N-[1-(2,6-dimethoxybenzyl)piperidin-4-yl]-4-sulfanylbutanamide | C18 H28 N2 O3 S | 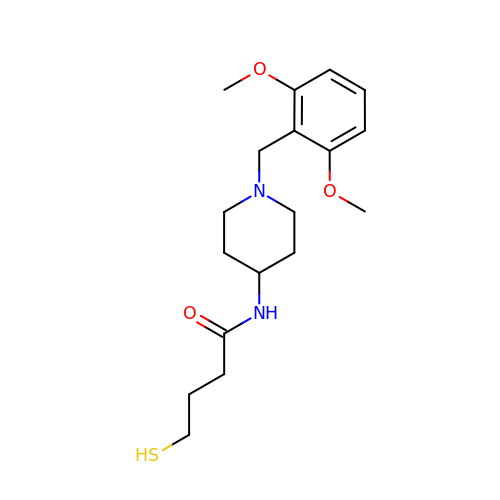MUDVORCZGBAHNA-UHFFFAOYSA-N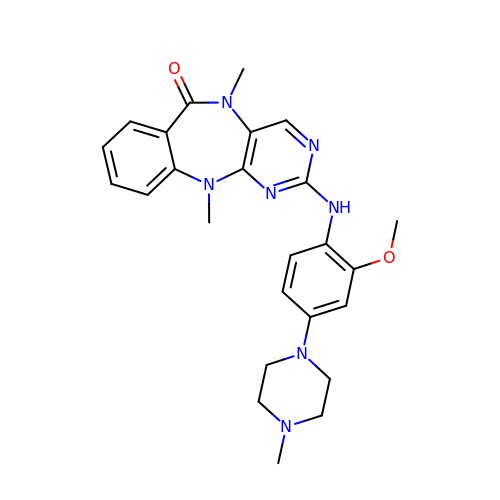2-{[2-methoxy-4-(4-methylpiperazin-1-yl)phenyl]amino}-5,11-dimethyl-5,11-dihydro-6H-pyrimido[4,5-b][1,4]benzodiazepin-6-one | C25 H29 N7 O2 | DDTPGANIPBKTNU-UHFFFAOYSA-N> MVDLRTQVLDVPVQETITKDNVPVRVN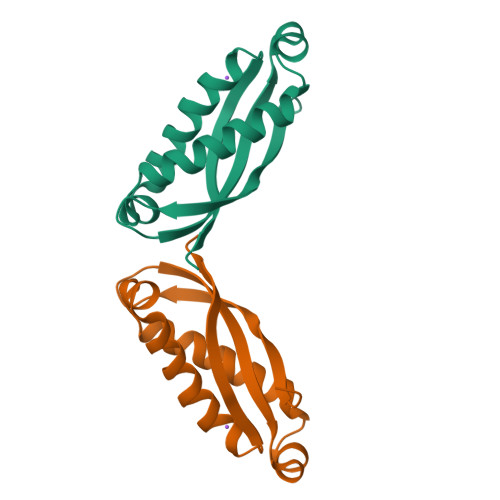AVVYFRVVDPVKAVTQVKNYIMATSQISQTTLRSVIGQAHLDELLSERDKLNMQLQRIIDEATDPWGIKVTAVEIKDVELPA>MPGSKSTAEQYAAYKQKMQKIADVRNAIAVLGWDQETYLPEKGAGFRGQQITTLSTIAHELFTAPELGSLLHELHHHPELDAVQQKNIALSLEDYDKNKKYPASLVAEISEATNQAYHAWIKARKANDYQVFEPALARMVELKRKETTVLGYEDHPYNALLNEYEKGANVDMLDTIFTEVKTALSPLLDDIAKQTPARRDFLHLHFDRDKQWQLGIDLLRQMGYDMSAGRQDISEHPFTTSFNPLDVRVTTRIDENDFSNMTWSCIHEGGHALYEQGLPTEQYGLPCGEAASLGIHESQSRLWENNVGRSLNFWKFQY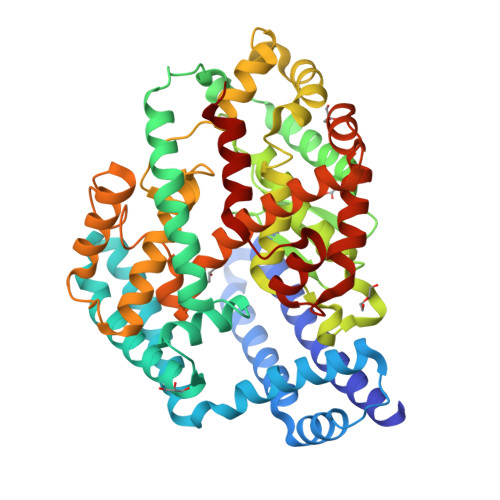PRIQALFPEQLGNVSLQEFYKAINHVQPSLIRTEADEITYHFHIMIRYEIEKGLIDGSISTKDLNKTWNDYYRQYLHVEVPNDTQGVLQDIHWSHGSFGYFPTYSLGSFYAAQFFTTAQKQVPDLDVSIASGNYQPLLEWLRNNIHPFGRFYTSNELCQKITGNPLQFSYFLDYAAGKFLRG[2x]>GPGSYNQALQGDPSFVLQIAEKEQELLASQETVQVLQMKVKRLEHLLQLKNVRIDDLSRRLQ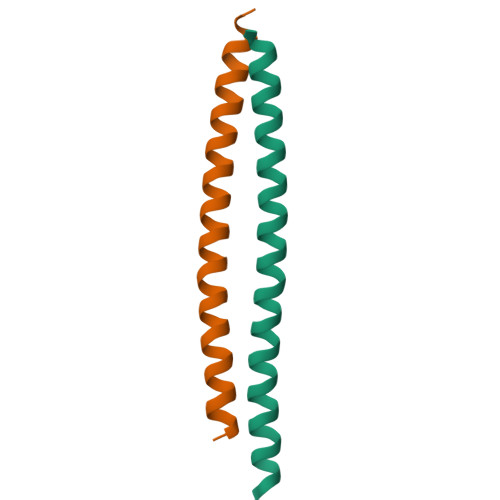QAERKQR[6x]>MNYAKEINALNNSLSDLKGDINVSFEFFPPKNEQMETMLWDSIHRLQTLHPKFVSVTYGANSGERDRTHGIVKRIKQETGLEAAPHLTGIDASPDELRQIAKDYWDSGIRRIVALRGDEPAGYEKKPFYAEDLVKLLRSVADFDISVAAYPEVHPEAKSAQADLINLKRKIDAGANHVIT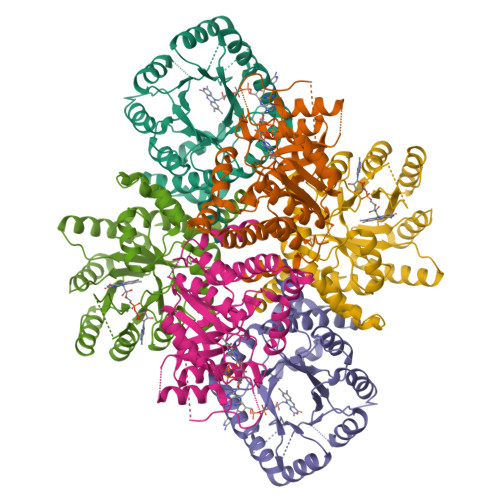QFFFDVERYLRFRDRCVMLGIDVEIVPGILPVTNFKQLGKMAQVTNVKIPSWLSQMYEGLDDDQGTRNLVAASIAIDMVKVLSREGVKDFHFYTLNRSELTYAICHILGVRPHHHHHH[3x]>GSHMTAPTVPVALVTGAAKRLGRSIAEGLHAEGYAVCLHYHRSAAEANALSATLNARRPNSAITVQADLSNVATAPVSGADGSAPVTLFTRCAELVAACYTHWGRCDVLVNNASSFYPTPLLRNDEDGHEPCVGDREAMETATADLFGSNAIAPYFLIKAFAHRVAGTPAKHRGTNYSIIN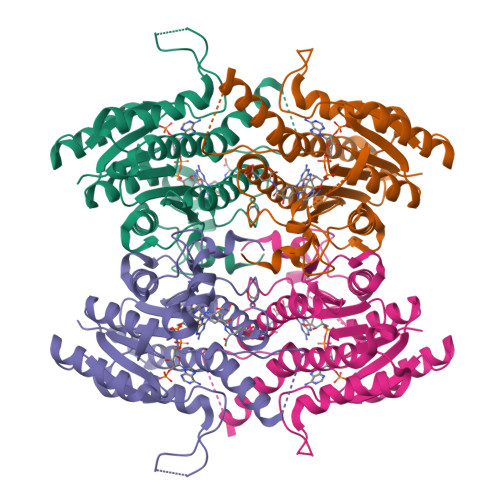MVDAMTNQPLLGYTIYTMAKGALEGLTRSAALELAPLQIRVNGVGPGLSVLVDDMPPAVWEGHRSKVPLYQRDSSAAEVSDVVIFLCSSKAKYITGTCVKVDGGYSLTRA[2x]>[2x]MRYRLAWLLHPALPSTFRSVLGARLPPPERLCGFQKKTYSKMNNPAIKRIGNHITKSPEDKREYRGLELANGIKVLLISDPTTDKSSAALDVHIGSLSDPPNIAGLSHFLQHMLFLGTKKYPKENEYSQFLSEHAGSSNAFTSGEHTNYYFDVSHEHLEGALDRFAQFFLSPLFDESAKDREVNAVDSEHEKNVMNDAWRLFQLEKATGNPKHPFSKFGTGNKYTLETRPNQEGIDVRQELLKFHSAYYSSNLMAVVVLGRESLDDLTNLVVKLFSEVENKNVPLPEFPEHPFQEEHLKQLYKIVPIKDIRNLYVTFPIPDLQKYYKSNPGHYLGHLIGHEGPGSLLSELKSKGWVNTLVGGQKEGARGFMFFIINVDLTEEGLLHVEDIILHMFQYIQKLRAEGPQEWVFQELKDLNA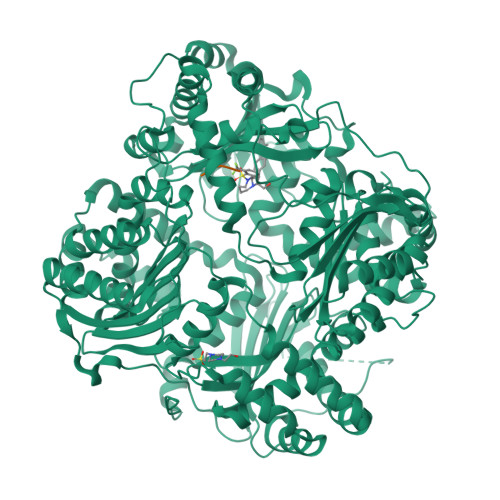VAFRFKDKERPRGYTSKIAGILHYYPLEEVLTAEYLLEEFRPDLIEMVLDKLRPENVRVAIVSKSFEGKTDRTEEWYGTQYKQEAIPDEVIKKWQNADLNGKFKLPTKNEFIPTNFEILPLEKEATPYPALIKDTAMSKLWFKQDDKFFLPKANLNFEFFSPFAYVDPLHSNMAYLYLELLKDSLNEYAYAAELAGLSYDLQNTIYGMYLSVKGYNDKQPILLKKIIEKMATFEIDEKRFEIIKEAYMRSLNNFRAEQPHQHAMYYLRLLMTEVAWTKDELKEALDDVTLPRLKAFIPQLLSRLHIEALLHGNITKQAALGIMQMVEDTLIEHAHTKPLLPSQLVRYREVQLPDRGWFVYQQRNEVHNNSGIEIYYQTDMQSTSENMFLELFAQIISEPAFNTLRTKEQLGYIVFSGPRRANGIQGLRFIIQSEKPPHYLESRVEAFLITMEKSIEDMTEEAFQKHIQALAIRRLDKPKKLSAESAKYWGEIISQQYNFDRDNTEVAYLKTLTKEDIIKFYKEMLAVDAPRRHKVSVHVLAREMDSNPVVGEFPAQNDINLSQAPALPQPEVIQNMTEFKRGLPLFPLVKPHINFMAAKL;>AAA[2x]2-AMINO-3-METHYL-1-PYRROLIDIN-1-YL-BUTAN-1-ONE | C9 H18 N2 O | 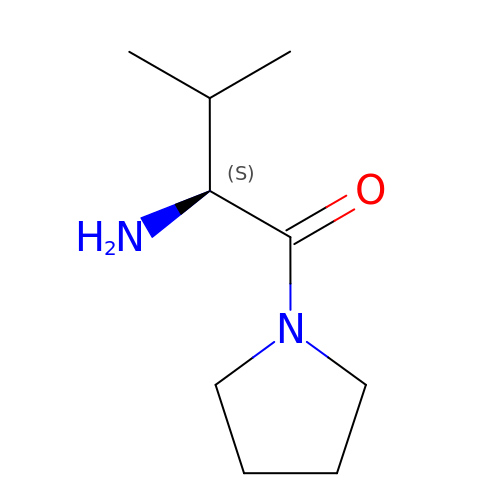IHBAVXVTGLANPI-QMMMGPOBSA-N>GMNRGKALQLVKPHLTEHRYQHTIGVMETAIDLAKLYGADQQKAE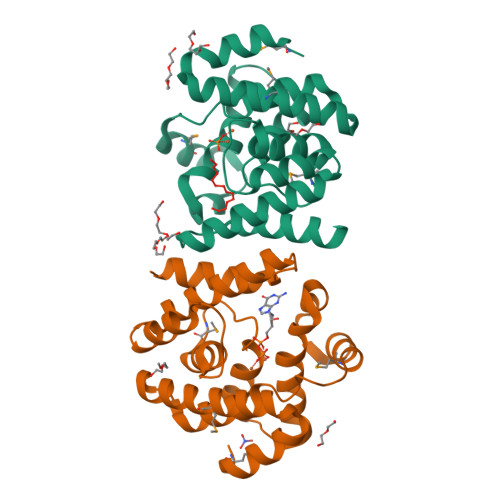LAAIFHDYAKFRDKNEMRTLIREKLSQQDILFYGDELLHAPCGAYYVREEVGIEDEDVLQAIRFHTTGRPNMSLLEKIIFLADYIEPNRQFPGVEKVRTQAKTDLNGAIISSLVNTITFLLKKNQPIYPDTLATYNQLLLEQK[2x]>HMKELKYDVLIIGGGFAGSSAAYQLSRRGLKILLVDSKPWNRIGDKPCGDAVSKAHFDKLGMPYPKGEELENKINGIKLYSPDMQTVWTVNGEGFELNAPLYNQRVLKEAQDRGVEIWDLTTAMKPIFEDGYVKGAVLFNRRTNEELTVYSKVVVEATGYSRSFRSKLPPELPITEDLDDKDADVAYREVLLTKEDIEDHDYLRIFIDQETSPGGYWWYFPKGKNKVNVGLGIQGGMGYPSIHEYYKKYLDKYAPDVDKSKLLVKGGALVPTRRPLYTMAWNGIIVIGDSGFTVNPVHGGGKGSAMISGYCAAKAILSAFETGDFSASGLWDMNICYVNEYGAKQASLDIFRRFLQKLSNDDINYGMKKKIIKEEDLLEASEKGDLHLSVADKAMRVISGLG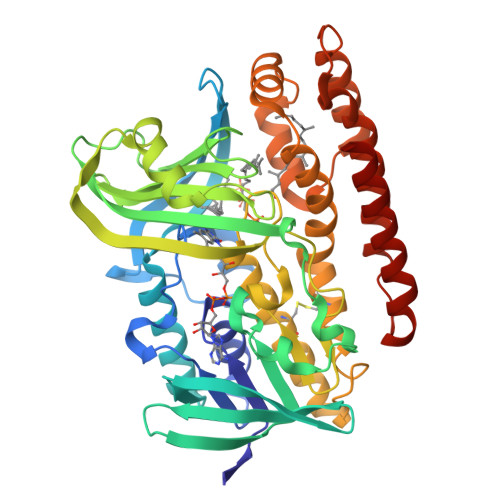RPSLLFKLKAVAESMKKIKELYLNYPRSPSSLGSWRREVDNVLTEFNKSLS[2x]>[2x]MKESRAKKFQRQHMDSDSSPSSSSTYCNQMMRRRNMTQGRCKPVNTFVHEPLLLVQLVCLQEKVTCKNGQGNCYK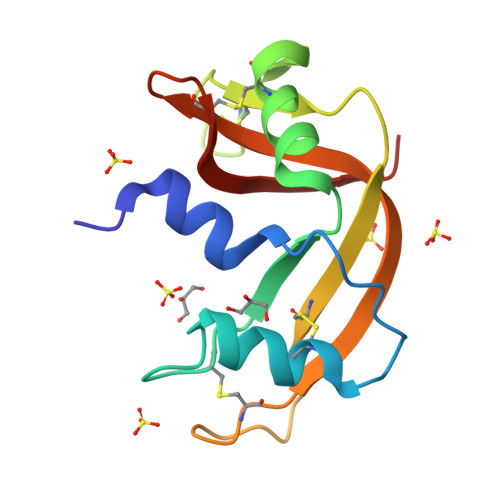SNSSMHITDCRLTNGSRYPNCAYRTSPKERHIIVACEGSPYVPVHFDASVEDST> DDNNTLYFYNWTEYVPPGLLEQFTKETGIKVIYSTYESNETMYAKLKTYKDGAYDLVVPSTYYVDKMRKEGMIQKIDKSKLTNFSNLDPDMLNKPFDPNNDYSIPYIWGATAIGVNGDAVDPKSVTSWADLWKPEYKGSLLLTDDAREVFQMALRKLGYSGNTTDPKEIEAAYNELKKLMPNVAAFNSDNPANPYMEGEVNLGMIWNGSAFVARQAGTPIDVVWPKEGGIFWMDSLAIPANA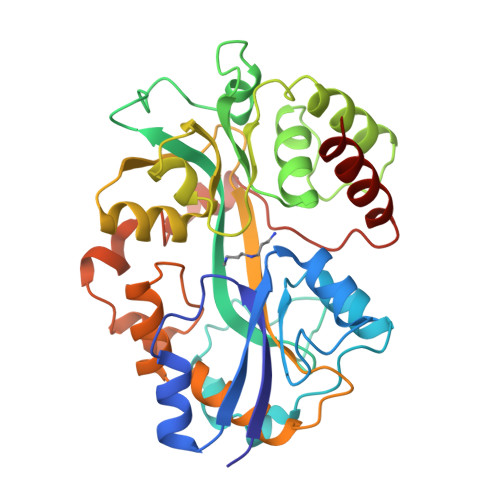KNKEGALKLINFLLRPDVAKQVAETIGYPTPNLAARKLLSPEVANDKTLYPDAETIKNGEWQNDVGAASSIYEEYYQKLKAGR>GCESVDFNLFNTIFSTHRGLSNTTSVITGAYPSTNKSDWSCNTRTGHLSGSGFGIGLYVQTPREQYQYDGSGAGGYTIAVSPIHVTNLTWELWIHRKWGVNSVVTVRLCRWWQFMSFNSTSHAADAGPTNAFECLINGSYPTHRNTGYMFGVTWYNDLVRIVFPPTVLEMQLDGLQWERVQFNSPVNAGHATRFNVVKDISTVLVETNSGGSVFRYSYCADGFVNGLQCKLRLFDIPPGVYSNSEVEYPTALYTVVHNMSACPERPDSYCGSNSCPFKRAVFSNCIVNYTTWVNPDQRDFQHLILPNGKFNPFTECNGLNRIVDGCVPGFVLRVGRGKAVNRTIVTPYLKPYECFGWSWNDNQDSIYDWWIADFVSTGAFVCESNPEAPKTGVCVTYTVEKVTFQGVLYESNFTFAQYYNLLYVGSQLRYVRILGKVYEVSSCFEASYDVLYRNNQSFGLLYRSFDCNQLHIKSARFVDRLLPSHNGTATVLGCLFNASYAPNDTMVNCTNPLGDGFCADLLGNVAVRRMTFEKHDTTYVAPVTNERYTEMPLDHQLILTEQFLQTTMPKFSVSCETYICDVSKACKNLLFRYGGFCQKVEADIRGAGILLDGDVSSLYSTIAAKTSSVVPTTDRFNVSQFFLPKTQSSANKYESRSAIEDLLFSKIETTGPGFYGDYYNCKKNAIQDLTCAQYHNGILVIPPIMD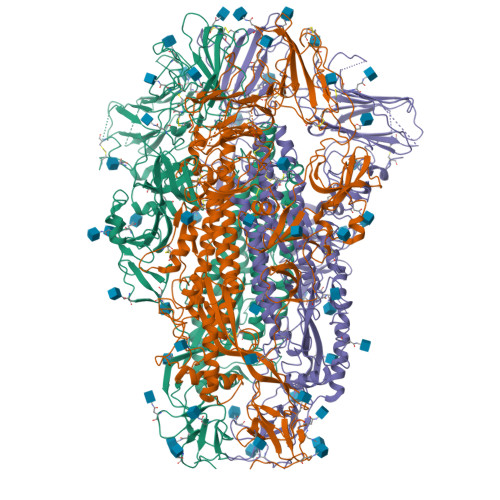AETLGMYGGIAAASVTLGIFGGQAGMATWSVAMAGRLNALGVVQNALVDDVNKLANGFNQLTASVSKLALTTSSALQAIQAVVNQNAAQVESLVSGITENFGAISTNFKVISQRLDKLEADVQMDRLINGRMNVLQLFVTNYKLKIAELRNTHRYVQSLINECVYAQSLRNGFCGQGLHVLSLMQNAPSGIMFFHYSLIPNNTITVKTTPGLCESDELGSKCIVAKDGVLVSANLSYWQWSPRNLYKPENLTFANVIAVSRGANYTTLNKTFDIP[3x]> NTKYNKEFLLYLAGFVDGDGSIIAQINPNASSKFKHRLRLTFYVTQKTQRRWFLDKLVDEIGVGYVRDSGSVSQYVLSEIAPLHNFLTQLQPFLKLKQKQANLVLKIIEQLPSAKASPAAFLEVCTWVDQIAALNDSATRKTTSETVAAVLD;> NTKYNKEFLLYLAGFVDGDGSIIAQIKP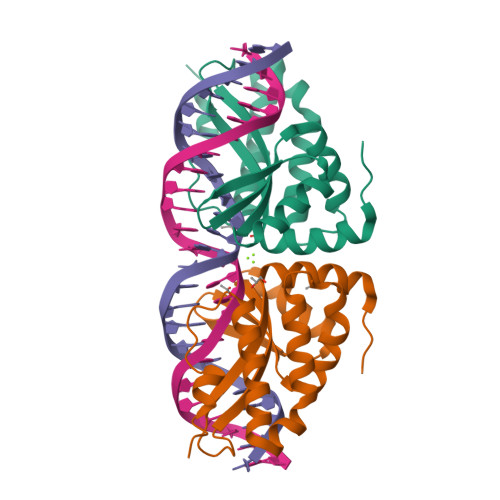RASNKFAHQLSLTFAVTQKTQRRWFLDKLVDEIGVGYVYDSGSVSDYRLSEIKPLHNFLTQLQPFLKLKQKQANLVLAIIEQLPSAKASPDAFLEVCTWVDQIAALNDSKTRATTSATVRAALD> GAPATVAEQGEDITSKKDRGVLKIVKRVGNGEETPMIGDKVYVHYKGKLSNGKKFDSSHDRNEPFVFSLGKGQVIKAWDIGVATMKKGEICHLLCKPEYAYGSAGSLPKIPSNATLF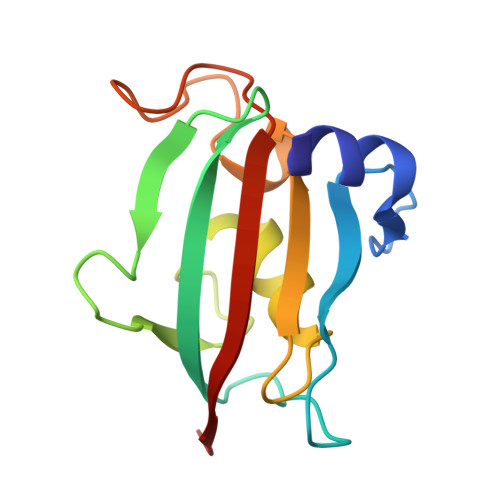FEIELLDFKGE>QQACSLTTERHPSLSWKKCTAGGQCQTVQASITLDSNWRWTHQVSGSTNCYTGNKWDTSICTDAKSCAQNCCVDGADYTSTYGITTNGDSLSLKFVTKGQHSTNVGSRTYLMDGEDKYQTFELLGNEFTFDVDVSNIGCGLNGALYFVSMDADGGLSRYPGNKAGAKYGTGYCDAQCPRDIKFINGEANIEGWTGSTNDPNAGAGRYGTCCSEMDIWEANNMATAFTPHPCTIIGQSRCEGDSCGGTYSNERYAGVCDPDGCDFNSYRQGNKTFYGKGMTVDTTKKITVVTQFLKDANGDLGEIKRFYVQDGKIIPNSESTIPGVEGNSITQDWCDRQKVAFGDIDDFNRKGG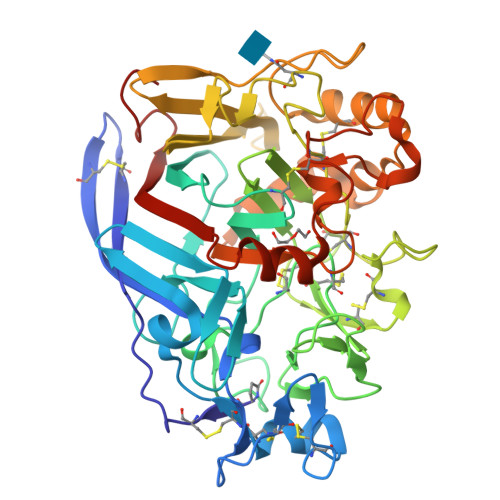MKQMGKALAGPMVLVMSIWDDHASNMLWLDSTFPVDAAGKPGAERGACPTTSGVPAEVEAEAPNSNVVFSNIRFGPIGSTVAGLPG[2x]>[2x]MNAKKRKGSAVERNIVSRLRDKGFAVVRAPAAGSKRKDPIPDIIALKNGVIILIEMKSRKDIEGKIYV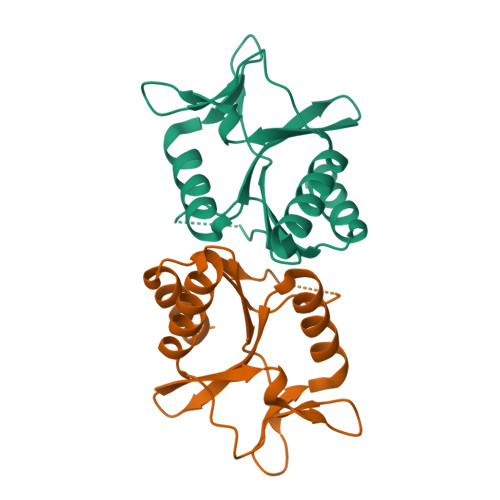RREQAEGIIEFARKSGGSLFLGVKKPGVLKFIPFEKLRRTETGNYVADSEIEGLDLEDLVRLVEAKISRTLDNFL(3-methoxy-5-pyridin-3-yl-phenyl)methyl 1~{H}-pyrazole-4-carboxylate | C17 H15 N3 O3 | 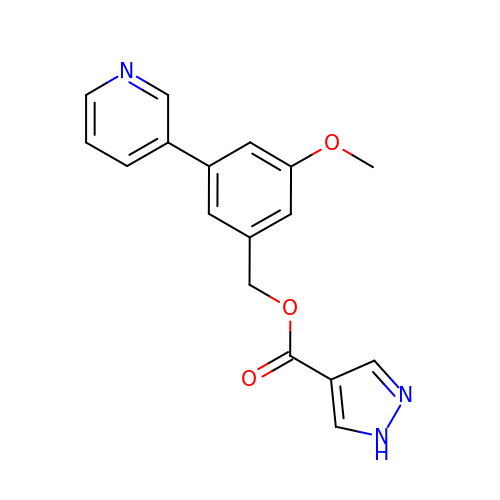JWEGKKOSKAIWMV-UHFFFAOYSA-N> PSPEQRVEIVPRDLRMKDKFLKHLTGPLYFSPKCSKHFHRLYHNTRDCTIPAYYKRCARLLTRLAVSPVCMEDKQGTDE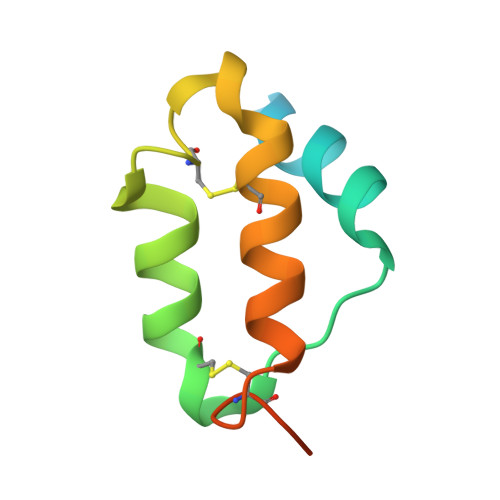VD2-(2-chloropyridin-4-yl)-4-methyl-1H-isoindole-1,3(2H)-dione 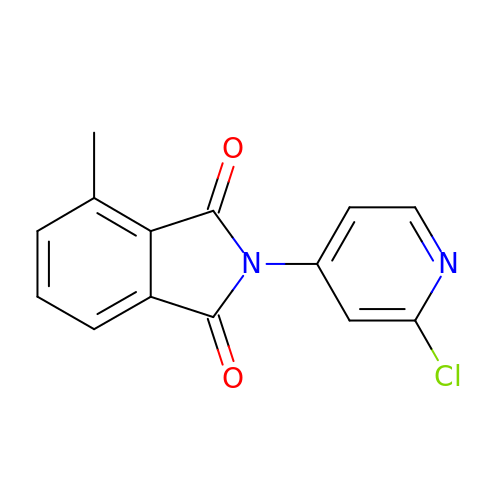| C14 H9 Cl N2 O2 | YDJMWNHJNJVVMM-UHFFFAOYSA-N>SNAMAGLKYEDAGVNIEAGNQAVERMKQHVKKTFTQDVLTGLGSFGSLYSLKNIINNYDDPVLVQSIDGVGTKTKVAVMCGKFENLGYDLFSAATNDIVVMGAKPITFLDYVAHDKLDPAIMEELVKGMSKACAECGVSLVGGETAEMPGVYQAGEIDMVGVITGIVDRKRIINGENIKEGDIVFGLSSSGLHTNGYSFARKLFFDVAGNKHTDTYPELEGKTIGDVLLEPHINYTNIIHDFLDNGVDIKGMAHITGGGFIENI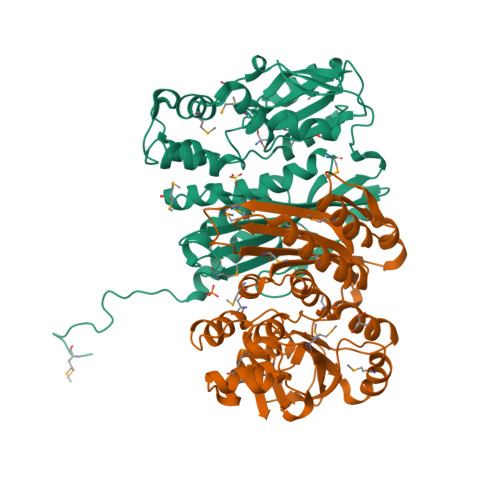PRVLPQGLGAQIDKDSFATPAIFKLMQRIGDISEFEMYRSFNMGIGMTIIASQDQFDKMQELAKKHTNTKLYQIGKITNSGKVEII[2x]>MTTVIDATMAYRFLEEATDSSSSSSSSKLESSPVDAVLFVGMSLVLGIASRHLLRGTRVPYTVALLVIGIALGSLEYGAKHNLGKIGHGIRIWNEIDPELLLAVFLPALLFESSFSMEVHQIKRCLGQMVLLAVPGVLISTACLGSLVKVTFPYEWDWKTSLLLGGLLSATDPVAVVALLKELGASKKLSTIIEGESLMNDGTAIVVFQLFLKMAMGQNSDWSSIIKFLLKVALGAVGIGLAFGIASVIWLKFIFNDTVIEITLTIAVSYFAYYTAQEWAGASGVLTVMTLGMFYAAFARTAFKGDSQKSLHHFWEMVAYIANTLIFILSGVVIAEGILDSDKIAYQGNSWRFLFLLYVYIQLSRVVVVGVLYPLLCRFGYGLDWKESIILVWSGLRGAVALALSLSVKQSSGNSHISKETGTLFLFFTGGIVFLTLIVNGSTTQFVLRLLRMDILPAPKKRILEYTKYEMLNKALRAFQDLGDDEELGPADWPTVESYISSLKGSEGELVHHPHNGSKIGSLDPKSLKDIRMRFLNGVQATYWEMLDEGRISEVTANILMQSVDEALDQVSTTLCDWRGLKPHVNFPNYYNFLHSKVVPRKLVTYFAVERLESACYISAAFLRAHTIARQQLYDFLGESNIGSIVINESEKEGEEAKKFLEKVRSSFPQVLRVVKTKQVTYSVLNHLLGYIENLEKVGLLEEKEIAHLHDAVQTGLKKLLRNPPIVKLPKLSDMITSHPLSVALPPAFCEPLKHSKKEPMKLRGVTLYKEGSKPTGVWLIFDGIVKWKSKILSNNHSLHPTFSHGSTLGLYEVLTGKPYLCDLITDSMVLCFFIDSEKILSLQSDSTIDDFLWQESALVLLKLLRPQIFESVAMQELRALVSTESSKLTTYVTGESIEIDCNSIGLLLEGFVKPVGIKEELISSPAALSPSNGNQSFHNSSEASGIMRVSFSQQATQYIVETRARAIIFNIGAFGADRTLHRRPSSLTPPRSSSSDQLQRSFRKEHRGLMSWPENIYAKQQQEINKTTLSLSERAMQLSIFGSMVNVYRRSVSFGGIYNNKLQDNLLYKKLPLNPAQGLVSAKSESSIVTKKQLETRKHACQLPLKGESSTRQNTMVESSDEEDEDEGIVVRIDSPSKIVFRNDL[2x]

Salt-overly-sensitive 1 (SOS1) is a unique electroneutral Na+/H+ antiporter at the plasma membrane of higher plants and plays a central role in resisting salt stress. SOS1, which is highly conserved in the phylae of the plant kingdom, is identified as the only Na+/H+ transporter that localizes at the plasma membrane and specifically exports Na+ by utilizing the electrochemical proton gradient generated by H+-ATPase6,7. SOS1 forms a homodimer and is composed of a TMD and an intracellular domain. Previous studies have shown that the C-terminus of SOS1 contains an autoinhibitory domain to keep the transporter in a resting state with basal activity.

However, superimposition of SOS1-ClassIV structure to the SOS1-ClassII structure gives rise to RMSDs of 1.5 Å for overall structure, indicating that two different SOS1 structures have been resolved. The structural comparison indicates that the dimerized SOS1-ClassIV harbors a distinct conformation to the 2.8-Å resolution SOS1 that the TMD undergoes significant conformational changes and the intracellular domains are nearly identical, supported by the RMSD values between these two structures are 2.0 Å and 0.7 Å for TMD and CTD, respectively. Taking a close look, the extracellular ends of TM helices from two protomers expand in opposing directions, except that the TM8 and TM9 remain unaltered, while the cytoplasmic ends of TM helices are superimposable. Therefore, we termed the SOS1-ClassIV structure as SOS1expand. Within the hydrophobic central cavity between dimerization domains, we found that the lipid molecules differently interact with the SOS1 in these two conformations. In both structures, four lipid molecules are determined at similar positions proximal to the 2-fold symmetrical axis. However, in the SOS1expand structure, an extra lipid is inserted into space between TM1 and TM3′ helices at the dimerization interface. Meanwhile, the side chain of Y270 on TM8′ is extruded in the SOS1expand structure to accommodate this lipid molecule. In the SOS1expand structure, two extra lipids were determined to be buried in the dimerization interface, leading to extracellular expansion of the TMD. However, the differences in bound lipids did not result in significant conformational changes in the intracellular ends of TM helices and in the intracellular domains.>MDNSHDSDSVFLYHIPCDNCGSSDGNSLFSDGHTFCYVCEKWTAGNEDTKERASKRKPSGGKPMTYNVWNFGESNGRYSALTARGISKETCQKAGYWIAKVDGVMYQVADYRDQNGNIVSQKVRDKDKNFKTTGSHKSDALFGKHLWNGGKKIVVTEGEIDMLTVMELQDCKYPVVSLGHGASAAKKTCAANYEYFDQFEQIILMFDMDEAGRKAVEEAAQVLPAGKVRVAVLPCKDANECHLNGHDREIMEQVWNAGPWIPDGVVSALSLRERIREHLSSEESVGLLFSGCTGINDKTLGARGGEVIMVTSGSGMGKSTFVRQQALQWGTAMGKKVGLAMLQESVEETAEDLIGLHNRVRLRQSDSLKREIIENGKFDQWFDELFGNDTFHLYDSFAEAETDRLLAKLAYMRSGLGCDVIILDHISIVVSASGESDERKMIDNLMTKLKGFAKSTGVVLVVICHLKNPDKGKAHEEGRPVSITDLRGSGALRQLSDTIIALERNQQGDMPNLVLVRILKCRFTGDTGIAGYMEYNKETGWLEPSSYSGEEESHSESTDWSNDTDF[6x];> MIVSDIEANALLESVTKFHCGVIYDYSTAEYVSYRPSDFGAYLDALEAEVARGGLIVFHNGHKYDVPALTKLAKLQLNREFHLPRENCIDTLVLSRLIHSNLKDTDMGLLRSGKLPGKRFGSHALEAWGYRLGEMKGEYKDDFKRMLEEQGEEYVDGMEWWNFNEEMMDYNVQDVVVTKALLEKLLSDKHYFPPEIDFTDVGYTTFWSESLEAVDIEHRAAWLLAKQERNGFPFDTKA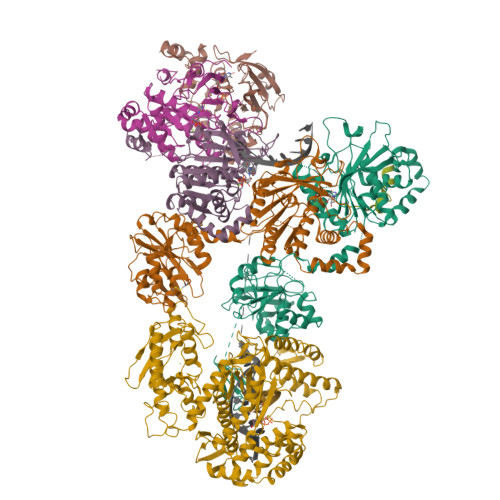IEELYVELAARRSELLRKLTETFGSWYQPKGGTEMFCHPRTGKPLPKYPRIKTPKVGGIFKKPKNKAQREGREPCELDTREYVAGAPYTPVEHVVFNPSSRDHIQKKLQEAGWVPTKYTDKGAPVVDDEVLEGVRVDDPEKQAAIDLIKEYLMIQKRIGQSAEGDKAWLRYVAEDGKIHGSVNPNGAVTGRATHAFPNLAQIPGVRSPYGEQCRAAFGAEHHLDGITGKPWVQAGIDASGLELRCLAHFMARFDNGEYAHEILNGDIHTKNQIAAELPTRDNAKTFIYGFLYGAGDEKIGQIVGAGKERGKELKKKFLENTPAIAALRESIQQTLVESSQWVAGEQQVKWKRRWIKGLDGRKVHVRSPHAALNTLLQSAGALICKLWIIKTEEMLVEKGLKHGWDGDFAYMAWVHDEIQVGCRTEEIAQVVIETAQEAMRWVGDHWNFRCLLDTEGKMGPNWAICH>[8x]ASQTITVGSWGGPGGNGWDEGSYTGIRQIELSYKEAIGSFSVIYDLNG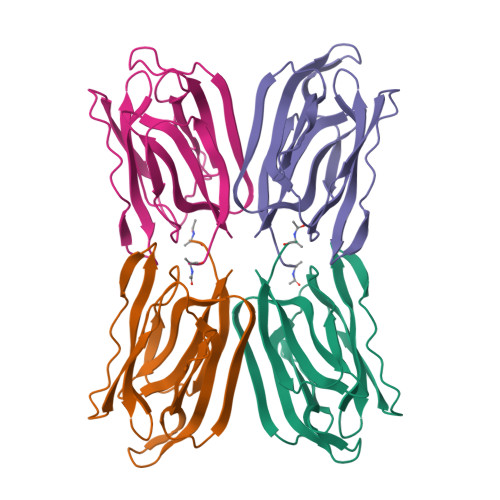DPFSGPKHTSKLPYKNVKIELKFPDEFLESVSGYTGPFSALATPTPVVRSLTFKTNKGRTFGPYGDEEGTYFNLPIENGLIVGFKGRTGDLLDAIGIHMSL>[6x]MLPRPSGTYAGLPIADYGDAPPLSTKTMFWRTSPEKLPPGAWEPAYLGSKDERVDGPSLQQVMRDQLKPYSEPRGLLPPQEILDAVCDAIENRLENTLEPQKPWTFKKACESLDKNTSSGYPYHKQKSKDWTGSAFIGDLGDQATHANNMYEMGKSMRPIYTAALKDELVKPDKIYGKIKKRLLWGSDLGTMIRAARAFGPFCDALKETCIFNPIRVGMSMNEDGPFIFARHANFRYHMDADYTRWDSTQQRAILKRAGDIMVRLSPEPDLARVVMDDLLAPSLLDVGDYKIVVEEGLPSGCPCTTQLNSLAHWILTLCAMVEVTRVDPDIVMQESEFSFYGDDEVVSTNLELDMVKYTMALRRYGLLPTRADKEEGPLERRQTLQGISFLRRAIVGDQFGWYGRLDRASIDRQL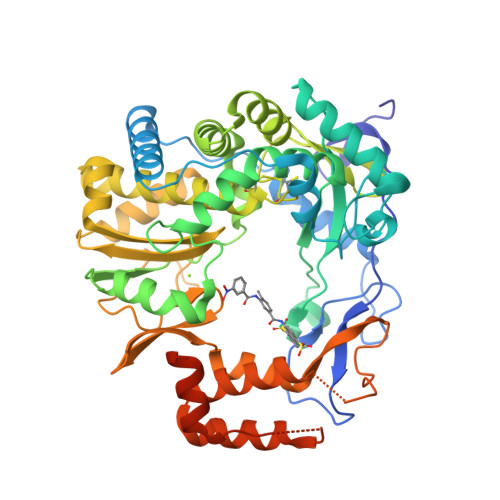LWTKGPNHQNPFETLPGHAQRPSQLMALLGEAAMHGEKYYRTVASRVSKEAAQSGIEMVVPRHRSVLRWVRFGTMDAETPQERSAVFVNEDELEHHHHHH>[3x]MQQLNPSEISALIKQRIGDLDTSATAKNEGTIVMVSDGIVRIHGLADAMYGEMIEFDGGLFGMALNLEQDSVGAVVLGNYLSLQEGQKARCTGRVLEVPVGPELLGRVVDALGNPIDGKGPIDAKLTDAVEKVAPGVIWRQSVDQPVQTGYKSVDTMIPVGRGQRELIIGDRQTGKTAMAIDAIIAQKNSGIKCVYVAIGQKQSTIANVVRKLEETGAMAYTTVVAAAAADPAAMQYLAPYSGCTMGEYFRDRGEDALIIYDDLSKQAVAYRQISLLLRRPPGREAYPGDVFYLHSRLLERASRVSAEYVEKFTNGAVTGKTGSLTALPIIETQAGDVSAFVPTNVISITDGQIFLETSLFNAGIRPAVNAGISVSRVGGSAQTKIIKKLSGGIRTALAQYRELAAFAQFASDLDEATRKQLEHGQRVTELMKQKQYAPYSIADQAVSVYASNEGYMADVEVKKIVDFDAALIAYFRSEYAPLMKQIDETGDYNKDIEAAIKAGIESFKATQTY;>MSSGRIIQIIGAVIDVEFERTSVPKIYDALQVDGTETTLEVQQQLGDGVVRTIAMGSTEGLKRGLTVTSTNAPISVPVGTATLGRIMDVLGRPIDEAGPVATEERLPIHRQAPSYAEQAASTDLLETGIKVIDLLCPFAKGGKVGLFGGAGVGKTVNMMELINNIAKAHSGLSVFAGVGERTREGNDFYHEMKDSNVLDKVAMVYGQMNEPPGNRLRVALTGLTMAEYFRDEKDENGKGRDVLLFVDNIYRYTLAGTEVSALLGRMPSAVGYQPTLAEEMGVLQERITSTKSGSITSIQAVYVPADDLTDPSPATTFAHLDATVVLSRDIASSGIYPAIDPLDSTSRQLDPLVVGQEHYEIARAVQNVLQRYKELKDIIAILGMDELAEEDKLVVYRARKIQRFFSQPFHVAEVFTGAPGKLVPLKETIRGFKGLLAGEYDHIPEQAFYMVGGIDEVIAKAEKL[3x];>[10x]MELTLGLVAIASAILIAFGALGTAIGFGLLGGRFLEAVARQPELAPQLQTRMFLIAGLLDAVPMIGVGIGLFFIFANPFVG;> MAAEEHALTSTEYIKHHLTNMTYGKMPDGTWKLAETAEEAHSMGFTAIHLDSMGWSIGLGVIFCLLFWIVARAANAGVPTKFQSAIEMIIEFVDSSVRDTFHGKSRLIAPLALTIFVWIFLMNLMDLIPVDWIPQVAAFVGANVFGMDPHHVYFKIVPSTDPNITLGMSLSVFVLILFYSIREKGVGGFVGELALNPFNPSNPVAKALLIPVNLILELVTFLARPISLALRLFGNMYAGELIFILIALLPFWIQWALSVPWAIFHILVITLQAFIFMMLTIVYLSMASEKH;>MNINLTLIGQAIAFAFFVAFCMKFVWPPLINAISERQRKIADGLNAAEKAKADLADAQAQVKQELDAAKAQAAQLIEQANRRAAQLIEEARTQAAAEGERIRQQAKEAVDQEINSAREELRQQVAALAVTGAEKILNQQVDAEAHNAMLSQLAAKL[2x];> MAELLTLARPYAKAAFAYASEQGATDNWSNALQVLSAAVQDEAFSAYLNRPELTPAEQVKLFAKVLGEDQSQAVSNFLTLLADNDRLVLLPEIAAEYEQLKSQNNNNVDVVIESAFPLTAEQEQLLKSALEKRFNSTVTVSVEVKPELIAGVVIRAGDQVIDDSALNKLEKMRTRLLA;> MATMQCDVVSVKESIYSGAVTMLIAKGAGGELGILPGHAPLVTLLQPGPIRVLLENGTEEIVYVSGGVLEVQPHVVTVLADTAIRADNLDEAAILEARKNAEQLLANQKSDLDSAAALAALAETAAQLETIRKIKNRAQ;> MANLKEIRAKVASIKSTQKITRAMQMVAASKMRRAQERMAQGRPYADNMRRVIAHLVQANPEYKHRYMVDRPVKRVGYIIVSSDRGLAGGLNINLFKKVVQHVKAQQEQSIEVQFALIGQKAVSFFKNYGGKVLGATTQIGDAPSLEQLTGSVQVMLDAFDKGELDRIYLVSNGFVNAMTQKPKVEQLVPLAPAEEGDDLNRTYGWDYIYEPEAEELLNGLLVRYIESMVYQGVIENVACEQSARMVAMKAATDNAGQLIKDLQLIYNKLRQAAITQEISEIVGGAAAV

F1Fo-ATP synthases are large, membrane-embedded macromolecular complexes that harness energy from the proton-motive force (pmf) and use it to synthesize ATP via a unique rotary mechanism. We solved the electron cryo-microscopy structure of the F1Fo–adenosine 5′-triphosphate (ATP) synthase from A. baumannii in three distinct conformational states. The A. baumannii ATP synthase has a subunit stoichiometry of α3β3γδεab2c10; its overall architecture resembles that of other bacterial and chloroplast ATP synthases. The rotating c-ring transfers torque to a central shaft comprising the ε- and γ-subunits, which protrude into the α3β3 hexamer, inducing conformational changes in the F1 nucleotide binding pockets, thus converting the rotary force into ATP synthesis.

State 1 was then used as a reference to build structures of the remaining two states. The central stalk is rotated by almost exactly 120o between each of the three conformational states suggesting common stable low-energy intermediate states in bacterial ATP synthases. Structural alignments of the γ-subunit between states revealed that the three states differ by almost exactly 120°.> MQASQFSAQVLDWYDKYGRKTLPWQIDKTPYKVWLSEVMLQQTQVATVIPYFERFMARFPTVTDLANAPLDEVLHLWTGLGYYARARNLHKAAQQVATLHGGKFPETFEEVAALPGVGRSTAGAILSLSLGKHFPILDGNVKRVLARCYAVSGWPGKKEVANKLWSLSEQVTPAVGVERFNQAMMDLGAMICTRSKPKCSLCPLQN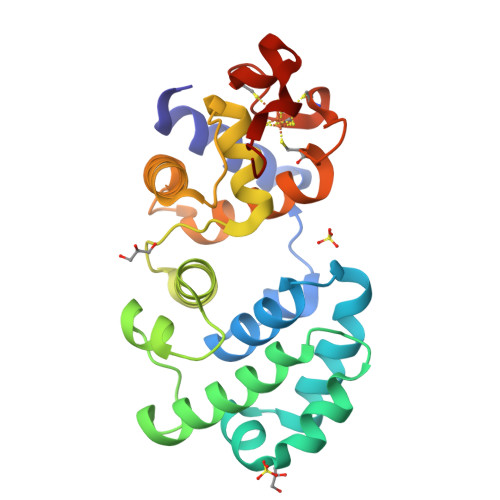GCIAAANNSWALYPGKKPK>MKIEEVKSTTKTQRIASHSHVKGLGLDESGLAKQAASGLVGQENAREACGVIVELIKSKKMAGRAVLLAGPPGTGKTALALAIAQELGSKVPFCPMVGSEVYSTEIKKTEVLMENFRRAIGLRIKETKEVYEGEVTELTPCETENPMGGYGKTISHVIIGLKTAKGTKQLKLDPSIFESLQKERVEAGDVIYIEANSGAVKRQGRCDTYATEFDLEAEEYVPLPKGDVHKKKEIIQDVTLHDLDVANARPQGGQDILSMMGQLMKPKKTEITDKLRGEINKVVNKYIDQGIAELVPGVLFVDEVHMLDIECFTYLHRALESSIAPIVIFASNRGNCVIRGTEDITSPHGIPLDLLDRVMIIRTMLYTPQEMKQIIKIRAQTEGINISEEALNHLGEIGTKTTLRYSVQLLTPANLLAKINGKDSIEKEHVEEISELFYDAKSSAKILADQQDKYMK[3x];>MATVTATTKVPEIRDVTRIERIGAHSHIRGLGLDDALEPRQASQGMVGQLAARRAAGVVLEMIREGKIAGRAVLIAGQPGTGKTAIAMGMAQALGPDTPFTAIAGSEIFSLEMSKTEALTQAFRRSIGVRIKEETEIIEGEVVEIQIDRPATGTGSKVGKLTLKTTEMETIYDLGTKMIESLTKDKVQAGDVITIDKATGKISKLGRSFTRARDYDAMGSQTKFVQCPDGELQKRKEVVHTVSLHEIDVINSRTQGFLALFSGDTGEIKSEVREQINAKVAEWREEGKAEIIPGVLFIDEVHMLDIESFSFLNRALESDMAPVLIMATNRGITRIRGTSYQSPHGIPIDLLDRLLIVSTTPYSEKDTKQILRIRCEEEDVEMSEDAYTVLTRIGLETSLRYAIQLITAASLVCRKRKGTEVQVDDIKRVYSLFLDESRSTQY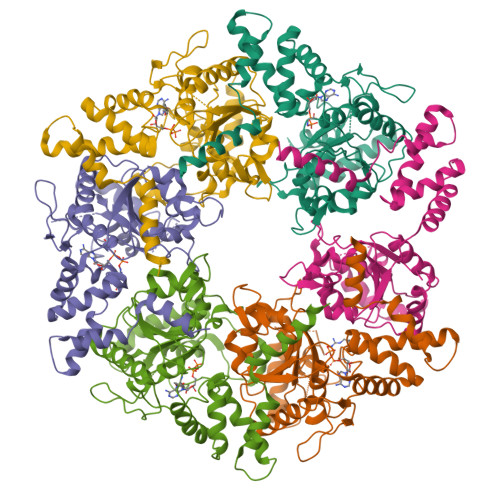MKEYQDAFLFNELKGETMDTS[3x]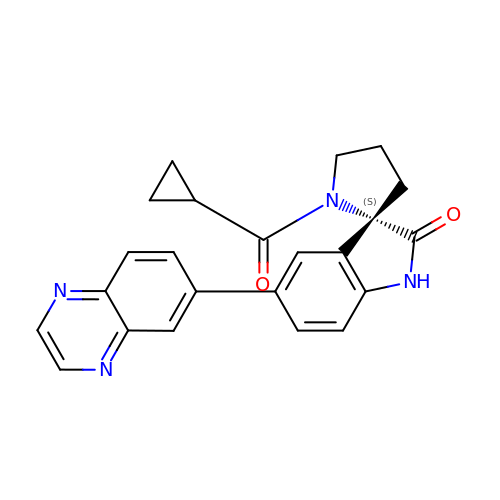(3S)-1'-(cyclopropanecarbonyl)-5-(quinoxalin-6-yl)spiro[indole-3,2'-pyrrolidin]-2(1H)-one | C23 H20 N4 O2 | PXPGVPPGCPSCSN-QHCPKHFHSA-N>MGSSHHHHHHHSSGLVPRGSHMDPVSVWGNTPLATVDPEIHDLIEKEKRRQCRGIELIASENFTSFAVIEALGSALTNKYSEGMPGNRYYGGNEYIDQIENLCRSRALQAFHLDAQSWGVNVQPYSGSPANFAAYTAVLNPHDRIMGLDLPSGGHLTHGYYTSGGKKISATSIYFESLPYKVNSTTGYIDYDRLEEKALDFRPKLIICGGSAYPRDWDYKRFREVADKCGALLLCDMAHTSGLVAAQEVNSPFEYCDIVTTTTHKSLRGPRAGMIFYRKGPKPPKKGQPEN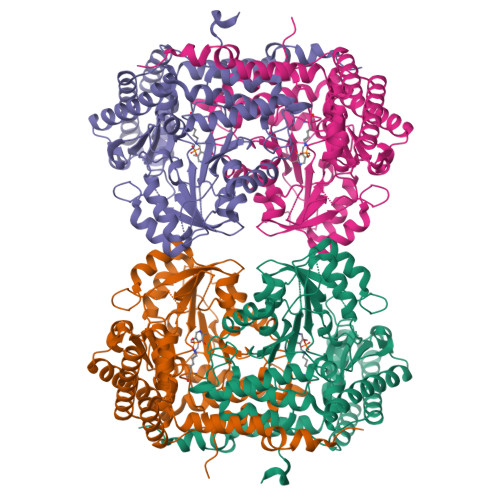AVYDFEDKINFAVFSSLQGGPHNHQIGALAVALKQAASPGFKAYAKQVKANAVALGKYLMGKGYSLVTGGTENHLVLWDLRPLGLTGNKVEKLCDLCNITVNKNAVFGDSSALAPGGVRIGAPAMTSRGLVEKDFEQIGEFLHRAVTLTLEIQKEHGKLLKDFNKGLVNNKAIEDLKADVEKFSALFDMPGFLVSEMKYKD[2x]> HP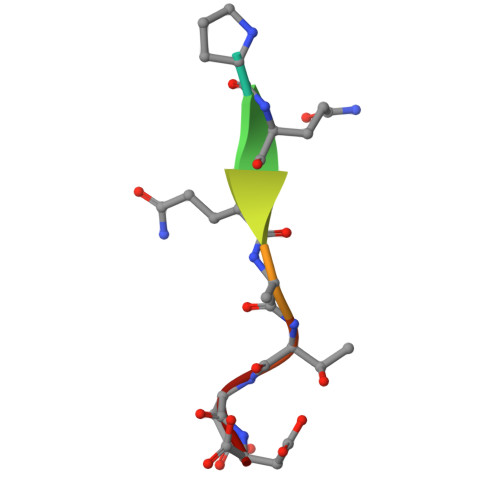QQATDD2-methyl-~{N}-[[5-(3-thiophen-2-yl-1,2,4-oxadiazol-5-yl)thiophen-2-yl]methyl]pyrazole-3-carboxamide 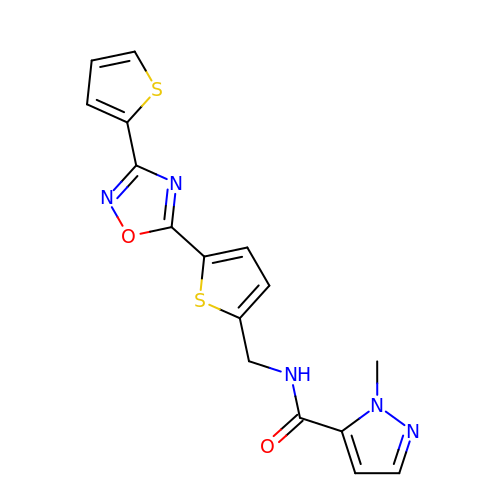| C16 H13 N5 O2 S2 | SIGJKWVCBZYUFS-UHFFFAOYSA-N> METGNKYIEKRAI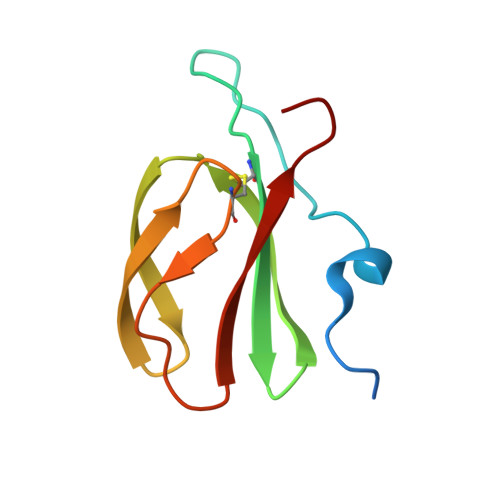DLSRERDPNFFDHPGIPVPECFWFMFKNNVRQDAGTCYSSWKMDMKVGPNWVHIKSDDNCNLSGDFPPGWIVLGKKRPGF>[4x]SGMATVMAATAAERAVLEEEFRWLLHDEVHAVLKQLQDILKEASLRFTLPGSGTEGPAKQENFILGSCGTDQVKGVLTLQGDALSQADVNLKMPRNNQLLHFAFREDKQWKLQQIQDARNHVSQAIYLLTSRDQSYQFKTGAEVLKLMDAVMLQLTRARNRLTTPATLTLPEIAASGLTRMFAPALPSDLLVNVYINLNKLCLTVYQLHALQPNSTKNFRPAGGAVLHSPGAMFEWGSQRLEVSHVHKVECVIPWLNDALVYFTVSLQLCQQLKDKISVFSSYWSYRPF

Rogdi is the human homolog of Drosophila melanogaster rogdi, and is a predicted leucine zipper protein of unknown function. The human Rogdi protein comprises 287 residues, and is highly conserved among species including fish, fly, frog, worm, and mouse. The crystal structure shows that Rogdi resembles a boomerang with an elongated curved structure comprising two distinct α and β domains. The α domain consists of four helices (H1 to H3, and H6) that form a left-handed four-helix bundle through van der Waals interactions.

Native crystals of the full-length protein grew in space group R3 and diffracted to 2.8 Å resolution using a synchrotron radiation source. Crystals of full-length Rogdi contain four molecules in the asymmetric unit. Interestingly, there are two conformations among the four molecules, with structural differences mainly at the N-terminus (residues 1–14), presumably due to crystal packing. Residues 1–14 in the two molecules fold into an α-helix (designated as RogdiH), extending the α-helix to residue 45, while the same regions in the remaining two molecules are unfolded and form a long loop (designated as RogdiL), suggesting that this region might be flexible in solution. The three loop regions (residues 64–68, 92–96, and 212–221) are disordered in the two RogdiH molecules; however, the electron density for RogdiL is relatively well ordered throughout the protein chain. The structure of the two RogdiH molecules and the two RogdiL molecules are almost identical, with RMSD values of 0.4 and 0.2 Å for all Cα atoms. Given that the N-terminal residues 1–11 are easily accessible and prone to proteolytic degradation, the non-paired region of H1 in the four-helix bundle (residues 1–14) might be flexible in solution. This is consistent with the structure of RogdiL, in which H1 helix residues 1–14 are disassociated from the helix and form a sharp bend due to steric hindrance by neighboring molecules in the crystal. The extended H1 helix in RogdiH engages in a parallel coiled-coil interaction with the adjacent H1 and H6 helices from the other molecule via crystal packing. In particular, a highly conserved hydrophobic patch comprising Leu 23, Ile 37, Leu 267, and Val 277 from H1 and H6 is exposed to the surface, suggesting that the hydrophobic surface generated by helices H1 and H6 could provide a platform for a protein–protein interaction module by conformational changes of the N-terminus into an extended H1 helix. The structures of full-length and truncated Rogdi are almost identical, with a root mean square deviation (RMSD) of 0.8 Å for all Cα atoms.>[2x]MELAAG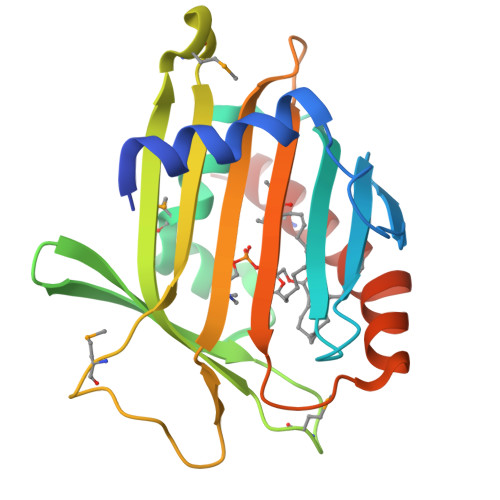SFSEEQFWEACAELQQPALAGADWQLLVETSGISIYRLLDKKTGLYEYKVFGVLEDCSPTLLADIYMDSDYRKQWDQYVKELYEQECNGETVVYWEVKYPFPMSNRDYVYLRQRRDLDMEGRKIHVILARSTSMPQLGERSGVIRVKQYKQSLAIESDGKKGSKVFMYYFDNPGGQIPSWLINWAAKNGVPNFLKDMARACQNYLKKT> MRGSHHHHHHTDLRADKASSIELKFDRNKGEVGDILIGTVRINNIKNFAGFQVNIVYDPKVLMAVDPETGKEFTSSTFPPGRTVLKNNAYGPIQIADNDPEKGILNFALAYSYIAGYKETGVAEESGIIAKIGFKILQKKSTAVKFQDTLSMPGAISGTQLFDWDGEVITGYEVIQPDVLSLGDEPF;> MNKPVIEGY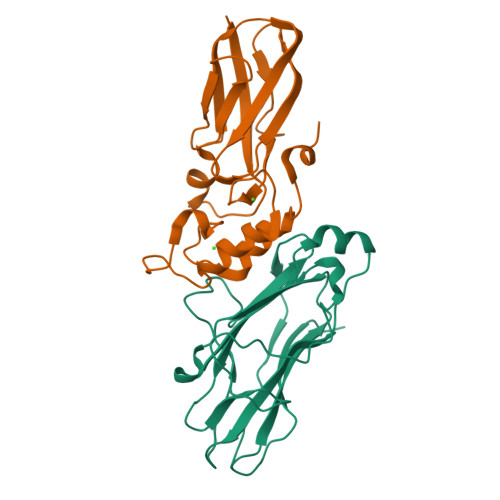KVSGYILPDFSFDATVAPLVKAGFKVEIVGTELYAVTDANGYFEITGVPANASGYTLKISRATYLDRVIANVVVTGDTSVSTSQAPIMMWVGDIVKDNSINLLDVAEVIRCFNATKGSANYVEELDINRNGAINMQDIMIVHKHFGATSSDYDAQLEHHHHHH In most cells, the detoxification of sulfite by oxidation to sulfate (Equation 1) is catalyzed by sulfite oxidizing enzymes (SOEs). Here, we have investigated an electron transfer complex involving the periplasmic SorT sulfite dehydrogenase from the α-Proteobacterium Sinorhizobium meliloti, which represents a structurally uncharacterized type of SOE, and its electron acceptor, the c-type cytochrome SorU. In S. meliloti the SorT sulfite dehydrogenase is part of a sulfite detoxification system that is induced in response to the degradation of sulfur containing substrates such as the organosulfonate taurine. Electrons derived from sulfite oxidation are passed on to the SorU cytochrome, and likely then to cytochrome oxidase, as S. meliloti is capable of sulfite respiration.

In order to investigate whether there are any structural reasons for these differences, we solved the crystal structure of SorT by molecular replacement and refined it to 2.4 Å resolution. The structure shows two homodimeric assemblies per asymmetric unit, which is in agreement with the quaternary structure as determined by MALLS. Unexpectedly however, within the SorT homodimer the protomers are oriented in a head-to-tail orientation, a subunit arrangement that has not been previously observed in structures of sulfite-oxidizing enzymes. Nevertheless, the fold of the SorT monomers is similar to those of other SOEs, comprising a central ‘SUOX-fold’ domain that harbors the Mo active site and a ‘dimerization’ domain. Within the SorT dimer, the subunit interface involves both the 'SUOX-fold' and the ‘dimerization’ domains, resulting in a buried surface area of ~1280 Å2 per monomer, which is approximately 9% of the solvent-accessible surface of each monomer. INSET: a closer view of the molybdenum binding-site: the molybdenum atom (green sphere) is coordinated by two dithioline ligands from the molybdopterin (yellow spheres), residue Cys 127, an axial oxo ligand and an equatorial hydroxo or water ligand (red spheres). SorT was crystallized by hanging drop vapor diffusion with drops consisting of equal volumes (2 μL) of protein and crystallization solution (0.1 M HEPES pH 7.5, 8% ethylene glycol, 0.1 M manganese (II) chloride tetrahydrate and 17.5% PEG 10,000) at 20°C. Crystals were cryoprotected in reservoir solution with 30% glycerol before flash-cooling in liquid nitrogen. The resulting model was refined by iterative cycles of amplitude based twin refinement (using twin operators H, K, L and –H, -K, L with estimated twin fractions of 0.495 and 0.505 respectively) within REFMAC, interspersed with manual inspection and correction against calculated electron density maps using COOT. The refinement of the model converged with residuals R = 0.208 and Rfree = 0.239.

>[4x]SKETKPLPDYVAWKDADALIVHSDKTLETKRSEFGTSIITPEEKLYIRNNVNTPPESILADRDGWKVEISGVKEPRTLTVAELKTLGLVTAATVLQCSGNGRKYFKDQLTGDQKMSGTPWTVGAAGCVIWSGVPLKAVVDALGGPAEGARFITGTGGEELPAGLDPKLLVVERSVPISNLDNVILAWEMNGRPLSLAHGGPLRMVVPGYSGVNNIKYVKAVAMTEVETDAKIQKTSYRVHALGEKGSPDQPSVWEQPVKSWITTPHEAAKAGQVQIAGVAFGGMNACKSVEVSVDGGQTWQEAEFIGPDLGRFAWRVFALSADLARGTYTLVSRATDTEGNVQPEETEMNGAGYGHNGWRAPAVKLTVA>[2x]QKPAACRCSRQDPKNRVNCGFPGITSDQCFTSGCCFDSQVPGVPW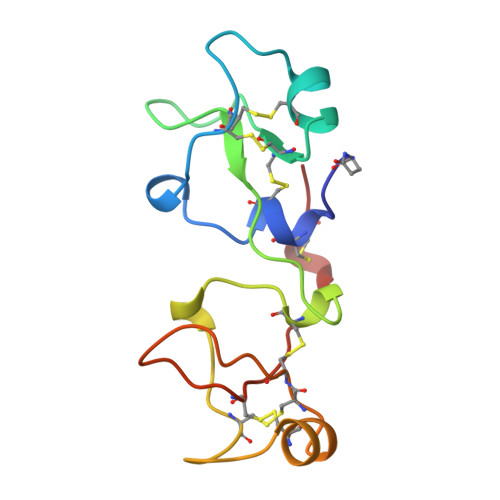CFKPLPAQESEECVMQVSARKNCGYPGISPEDCAARNCCFSDTIPEVPWCFFPMSVEDCHY>ADDYATTRYPIVLVHGLTGTDKYAGVLEYWYGIQEDLQQHGATVYVANLSGFQSDDGPNGRGEQLLAYVKTVLAATGATKVNLVGHSQGGLTSRYVAAVAPDLVASVTTIGTPHRGSEFADFVQGVLAYDPTGLSSSVIAAFVNVFGILTSSSHNTNQDALASLKTLTTAQAATYNQNYPSAGLGAPGSCQTGAPTETVGGNTHLLYSWAGTAIQPTLSVFGVTGATDTSTIPLVDPANALDPSTLALFGTGTVMINRGSGQN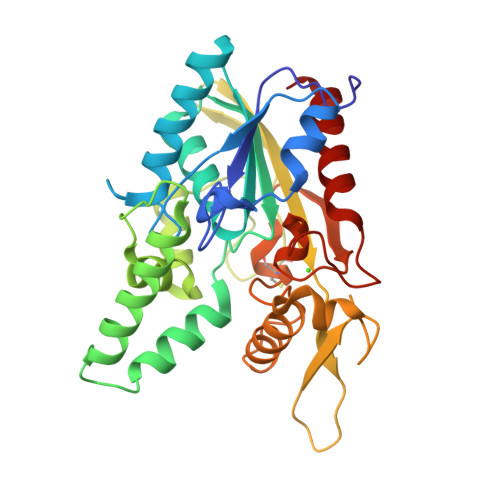DGLVSKCSALYGQVLSTSYKWNHIDEINQLLGVRGAFAEDPVAVIRTHANRLKLAGV[4x]>SQANLMRLKSDLFNRSPMYPGPTKDDPLTVTLGF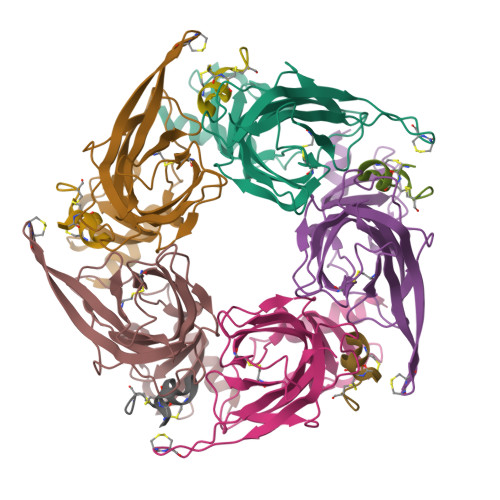TLQDIVKVDSSTNEVDLVYYEQQRWKLNSLMWDPNEYGNITDFRTSAADIWTPDITAYSSTRPVQVLSPQIAVVTHDGSVMFIPAQRLSFMCDPTGVDSEEGVTCAVKFGSWVYSGFEIDLKTDTDQVDLSSYYASSKYEILSATQTRQVQHYSCCPEPYIDVNLVVKFRERR[5x];>GCCSHPACNVAHPEICX[5x]>[6x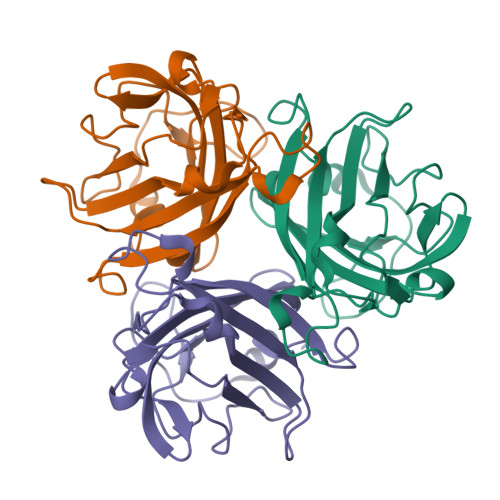]MRGSHHHHHHGSPPAAPITLWTGPGPSINGFINDTPVIRCFICLTRDSNLVTVNASFVGEGGYRIVSPTQSQFSLIMEFDQFGQLMSTGNINSTTTWGEKPWGNNTVQPRPSHTWKLCMPNREVYSTPAATISRCGLDSIAVDGAPSRSIDCMLIINKPKGVATYTLTFRFLNFNRLSGGTLFKTDVLTFTYVGENQ> IDPRFPHHHPRPQSFWEARAKALESLLIEKGHLSSDAIERVIKHYEHELGPMNGAKVVAKAWTDPAFKQRLLEDSETVLRELGYYGLQGEHIRVVENTDTVHNVVVCTLCSCYPWPLLGLPPSWYKEPAYRARVVKEPRQVLKEFGLDLPDSVEIRVWDRSSEIRFMVLPQRPEGTEGMTEEELAKLVTRDSMIGVAKIEPPKVTVG;> MNGIHDVGGMDGFGKVMYVKEEEDIYFTHDWERLAFGLVAGCKAQGLGMKAFDEFRIGIELMRPVDYLTSSYYGHWIATVAYNLVDTGVLDEKELDERTEVFLKKPDTKIPRREDPALVKLVEKALYDGLSPLREISASPRFKVGERIKAKNIHPTGHTRFPRYARDKYGVIDEVYGAHVFPDDAAHRKGENPQYLYRVRFEAEELWGYKQKDSVYIDLWESYME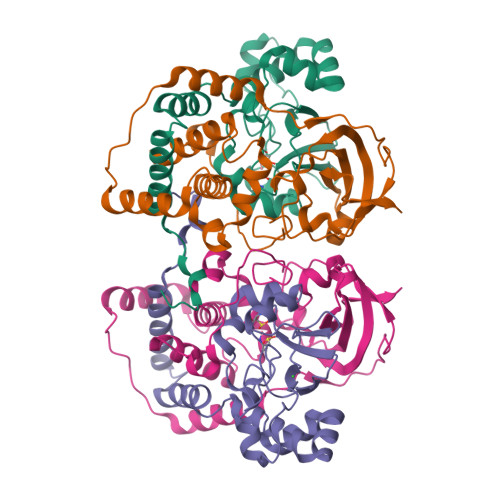PVSH>[4x]MGSHHHHHHSSGLVPRGSHMSEPQRLKPVFPQDPKWPGEGSSRVPFWAYTREDLYKRELER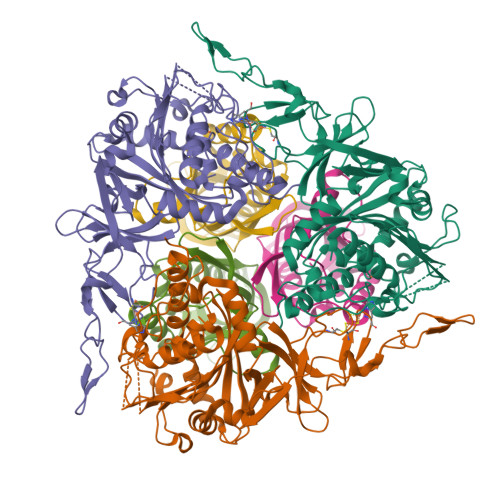LFYANHWCYVGLEAEIPNPGDFKRTVIGERSVIMVRDPDGGINVVENVCAHRGMRFCRERHGNAKDFFCPYHQWNYSLKGDLQGVPFRRGVKQDGKVNGGMPKDFKLEEHGLTKLKVAARGGAVFASFDHDVEPFEEFLGPTILHYFDRVFNGRKLKILGYRRQRIPGNWKLMQENIKDPYHPGLLHTWFSTFGLWRADNKSELKMDAKFRHAAMISTRGQGGKNEEVVSGVDSFKEQMKVNDPRLLDIVPEPWWGGPTAVMTTIFPSVIIQQQVNSVSTRHIQPNGHGSFDFVWTHFGFEDDNEEWTQRRLIQANLFGPAGFVSADDGEVIEWSQEGFEQKPTHRTVIEMGGHEIGDTDHMVTETLIRGMYDYWRKVMGE;>MVDFKTYFELLNLYSDYAMVCDSANWEKWPDFFIETGTYRLQPRENFEQGLPLCLLALESKAMIRDRVYGVKETMYHDPYYQRHIVGTPRVLSVERDADGERITAEASYAVIRTKYDGDSTIFNAGYYRDVIVRTPEGLKLKSRLCVYDSEMIPNSVIYPI[4x]In this study, we experimentally determined the function of a putative protein, as a novel alginate lyase (PsAly), whose gene is found beside two characterised chitinase genes (chiC and chiD) in the genome. Bacterial alginate lyases can degrade alginate into oligosaccharides or monosaccharides. Lyases catalyse a β-elimination reaction of glycoside bonds to yield a 4,5-unsaturated sugar, 4-deoxy-L-erythro-hex-4-enopyranosyluronic acid, at the non-reducing end11. PsAly preferentially degraded the glycosidic bond of PM over PG and MG.

To determine the structural characteristics of PsAly, the crystal structure of the enzyme was determined at an ultra-high resolution of 0.89 Å using the single-wavelength anomalous diffraction of selenium (Se-SAD). The refined model comprised 298 residues (Ala36 to Ala333) for one protein molecule in an asymmetric unit. PsAly folds into a right-handed β-helix structure comprising 10 β-stranded coils and one α-helix cap at the N-terminus, with overall dimensions of 26 × 28 × 52 Å. A single disulphide bond was formed between Cys42 and Cys47, linking the first β-strand to the first α-helix at the N-terminal cap structure. The long cleft from the N-terminus to the C-terminus is formed by the external surface of PB1, T1, and T3, of approximately 20 × 10 × 15 Å. After refinements with replacement of these ions on the sites, the Fo–Fc electron density map showed strong negative peaks in the presence of calcium ions on the sites, while the map in the presence of the sodium ions showed no such strong negative peaks. The residues Tyr184 and Lys221 were located near the first cation binding site. Considering the position of the ligand and the mutagenic results, the sidechains of Tyr184 and/or Lys221 are the most likely candidates for the base and/or acid catalysts.

> MATRTISCATASCLQSALKNAKPGDDIVLAEGVTFKGSFKAEASGTASQPITIRSAGSVNPAVLSGYSTGGGYSLYVTGDYWNITGLKMTGALKGIMLDHANHVQMDGLEIYDIGDEGVHFRDGSSDNIIRNSHIYNTGLIEAGFGEGIYVGSDKGKWATYNKSADRNVISGVRIGPGVAAEHIDIKEGTVGTIVENSVFNGTGITGANYADSFIDVKGNDAVIRNNIGYRNGNSNIVDAFQVHVQVAGWGQNATFTGNTVYLDQAAPYVVNAVGDATASAAGNQRYPAGNLYQGHVNALEHHHHHH>[3x]MSANVQEAANAAIEPASFVKVPMPEPPSSLQQLINDWQLIKHREGGYFKETDRSPYTMEVEKPVNGGSGNTEMVTRNQSTLIYYLLTPDSPIGKFHKNINRIIHILQRGKGQYVLVYPD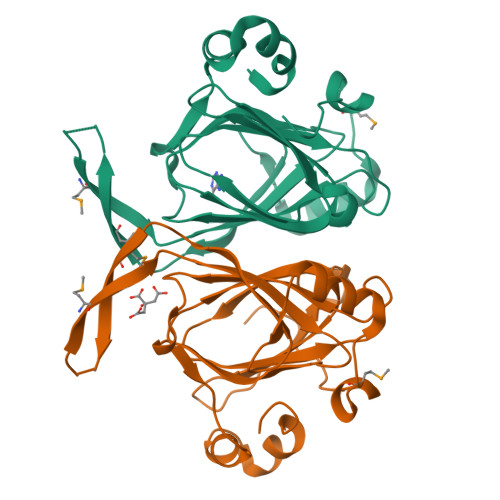GQVKSFKVGFDYKNGEVSQWVVPGGVFKASFLLPNEEFDNGFLISEVVVPGFDFEDHTFLKGEDELKHLVGPEKAAELAFLAHH> MTDT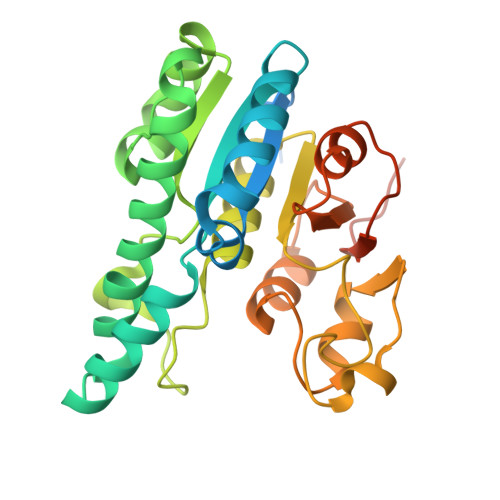TNSIKHVISPLARQTLQDRDLTRPVAGKRPIRLLPWLQVVKIGGRVMDRGADAILPLVEELRKLLPEHRLLILTGAGVRARHVFSVGLDLGLPVGSLAPLAASEAGQNGHILAAMLASEGVSYVEHPTVADQLAIHLSATRAVVGSAFPPYHHHEFPGSRIPPHRADTGAFLLADAFGAAGLTIVENVDGIYTADPNGPDRGQARFLPETSATDLAKSEGPLPVDRALLDVMATARHIERVQVVNGLVPGRLTAALRGEHVGTLIRTGVRPAENLYFQGSAWSHPQFEK> MRGSHHHHHHGSGTDITNQLTNVTVGIDSGTTVYPHQAGYVKLNYGFSVPNSAVKGDTFKITVPKELNLNGVTSTAKVPPIMAGDQVLANGVIDSDGNVIYTFTDYVNTKCDVKATLTMPAYIDPENVKKTGNVTLATGIGSTTANKTVLVDYEKYGKFYNLSIKGTIDQIDKTNNTY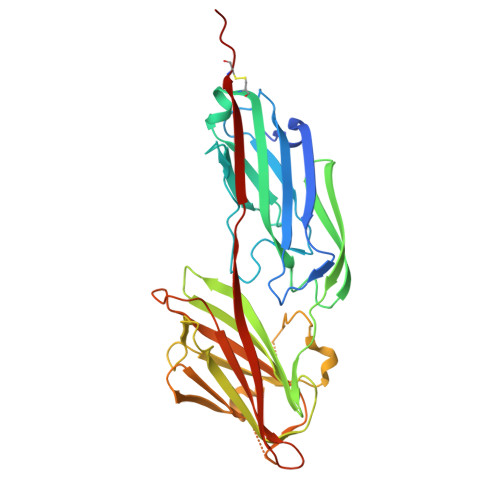RQTIYVNPSGDNVIAPVLTGNLKPNTDSNALIDQQNTSIKVYKVDNAADLSESYFVNPENFEDVTNSVNITFPNPNQYKVEFNTPDDQITTPYIVVVNGHIDPNSKGDLALRSTLYGYNSNIIWRSMSWDNEVAFNNGSGSGDGIDCPVVP>MYGKIIFVLLLSEIVSISASSTTGVAMHTSTSSSVTKSYISSQTNDTHKRDTYAATPRAHEVSEISVRTVYPPEEETGERVQLAHHFSEPEITLIIFGVMAGVIGTILLISYGIRRLIKKSPSDVKPLPSPDTDVPLSSVEIENPETSDQ[2x];>[2x]MEELQDDYEDMMEENLEQEEYEDPDIPESQMEEPAAHDTEATATDYHTTSHPGTHKVYVELQELVMDEKNQELRWMEAARWVQLEENLGENGAWGRPHLSHLTFWSLLELRRVFTKGTVLLDLQETSLAGVANQLLDRFIFEDQIRPQDREELLRALLLKHSHAGELEALGGVKPAVLTRSGDPSQPLLPQHSSLETQLFCEQGDGGTEGHSPSGILEKIPP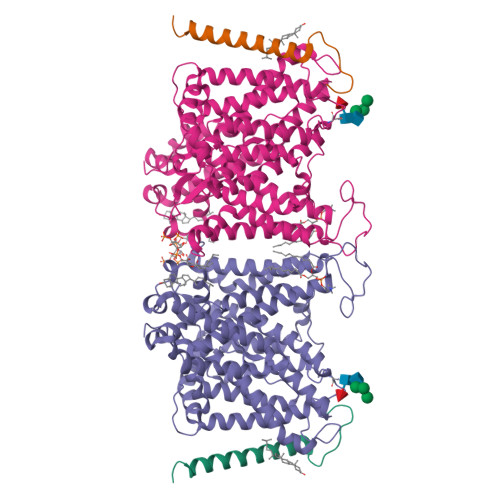DSEATLVLVGRADFLEQPVLGFVRLQEAAELEAVELPVPIRFLFVLLGPEAPHIDYTQLGRAAATLMSERVFRIDAYMAQSRGELLHSLEGFLDCSLVLPPTDAPSEQALLSLVPVQRELLRRRYQSSPAKPDSSFYKGLDLNGGPDDPLQQTGQLFGGLVRDIRRRYPYYLSDITDAFSPQVLAAVIFIYFAALSPAITFGGLLGEKTRNQMGVSELLISTAVQGILFALLGAQPLLVVGFSGPLLVFEEAFFSFCETNGLEYIVGRVWIGFWLILLVVLVVAFEGSFLVRFISRYTQEIFSFLISLIFIYETFSKLIKIFQDHPLQKTYNYNVLMVPKPQGPLPNTALLSLVLMAGTFFFAMMLRKFKNSSYFPGKLRRVIGDFGVPISILIMVLVDFFIQDTYTQKLSVPDGFKVSNSSARGWVIHPLGLRSEFPIWMMFASALPALLVFILIFLESQITTLIVSKPERKMVKGSGFHLDLLLVVGMGGVAALFGMPWLSATTVRSVTHANALTVMGKASTPGAAAQIQEVKEQRISGLLVAVLVGLSILMEPILSRIPLAVLFGIFLYMGVTSLSGIQLFDRILLLFKPPKYHPDVPYVKRVKTWRMHLFTGIQIICLAVLWVVKSTPASLALPFVLILTVPLRRVLLPLIFRNVELQCLDADDAKATFDEEEGRDEYDEVAMPV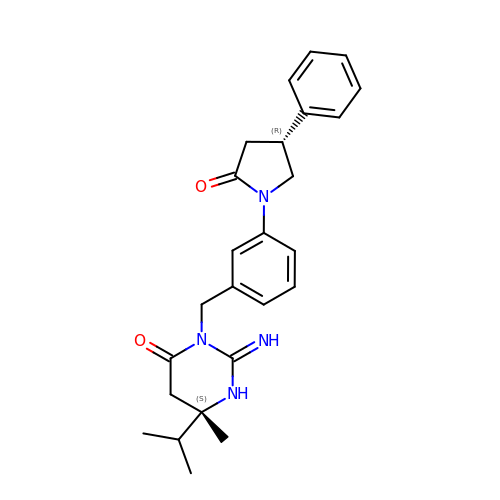(2Z,6S)-2-imino-6-methyl-3-{3-[(4R)-2-oxo-4-phenylpyrrolidin-1-yl]benzyl}-6-(propan-2-yl)tetrahydropyrimidin-4(1H)-one | C25 H30 N4 O2 | VBYHYTJHKFQNCE-CPJSRVTESA-N> MASQPNSSAKKKEEKGKNIQVVVRCRPFNLAERKASAHSIVECDPVRKEVSVRTGGLADKSSRKTYTFDMVFGASTKQIDVYRSVVCPILDEVIMGYNCTIFAYGQTGTGKTFTMEGERSPNEEYTWEEV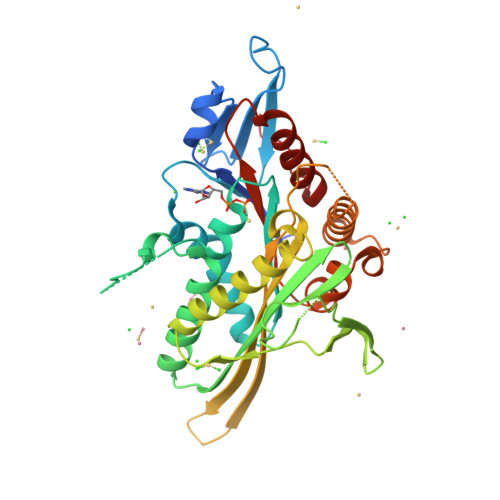PLDGIIPRTLHQIFEKLTDNGTEFSVKVSLLEIYNEELFDLLNPSSDVSERLQMFDDPRNKRGVIIKGLEEITVHNKDEVYQILEKGAAKRTTAATLMNAYSSRSHSVFSVTIHMKETTIDGEELVKIGKLNLVDLAGSENIGRSGAVDKRAREAGNINQSLLTLGRVITALVERTPHVPYRESKLTRILQDSLGGRTRTSIIATISPASLNLEETLSTLEYAHRAKNILNKPEVNQK> HHHHHHGACPSQCSCSGTTVNCKSKSLASVPAGIPTTTRVLYLNDNQITKLEPGVFDRLVNLQTLWLNNNQLTSLPAGLFDSLTQLTILALDSNQLQALPVGVFGRLVDLQQLYLGSNQLSALPSAVFDRLVHLKELLMCCNKLTELPRGIERLTHLTHLALDQNQLKSIPHGAFDRLSSLTHAYLFGN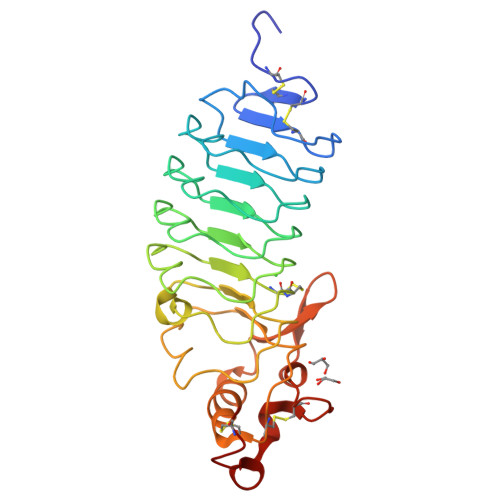PWDCECRDIMYLRNWVADHTSIVMRWDGKAVNDPDSAKCAGTNTPVRAVTEASTSPSKCP> SFRTDKKPDP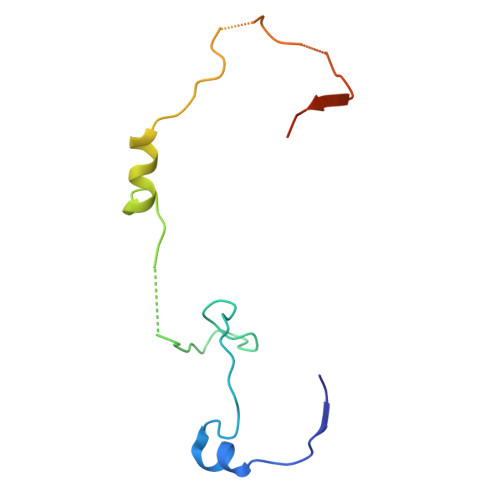ANWEYKSLYRGDIARYKRKGDSCLGINPKKQCISWEGTSTEKKHSRKQVERYFTKKSVGLMNIDGVAISSKTEPPSSEPISFIPVKDLEDAAPVT> GGSRCQRDHLSTKLIPTEVPADLIRAVTCQVCDHLLSDPVQSPCRHLFCRLCIIRYTHALGPNCPTCNQHLNPSHLIKPAKFFLAT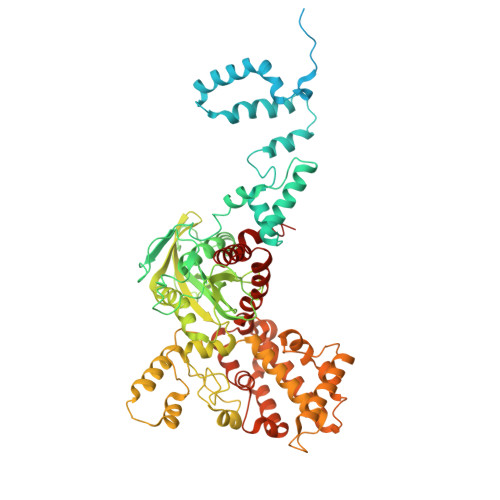LSSLPLLCPSEECSDWVRLDSFREHCLNHYREKESQEEQTPSEQNLDGYLPVNKGGRPRQHLLSLTRRAQKHRLRDLKNQVKTFAEKEEGGDVKSVCLTLFLLALRAGNEHKQADELEAMMQGRGFGLHPAVCLAIRVNTFLSCSQYHKMYRTVKATSGRQIFQPLHTLRNAEKELLPGFHQFEWQPALKNVSTSWDVGIIDGLSGWTVSVDDVPADTISRRFRYDVALVSALKDLEEDIMEGLRERALDDSMCTSGFTVVVKESCDGMGDVSEKHGSGPAVPEKAVRFSFTIMSISIRLEGEDDGITIFQEQKPNSELSCRPLCLMFVDESDHETLTAILGPVVAERKAMMESRLIISVGGLLRSFRFFFRGTGYDEKMVREMEGLEASGSTYICTLCDSTRAEASQNMVLHSITRSHDENLERYEIWRKNPFSESADELRDRVKGVSAKPFMETQPTLDALHCDIGNATEFYKIFQDEIGEVYQKPNPSREERRRWRSTLDKQLRKKMKLKPVMRMNGNYARRLMTREAVEAVCELVPSEERREALLKLMDLYLQMKPVWRSTCPSRDCPDQLCQYSYNSQQFADLLSSMFKYRYDGKITNYLHKTLAHVPEIVERDGSIGAWASEGNESGNKLFRRFRKMNARQSKTFELEDILKHHWLYTSKYLQKFMEAHKNS5-{[4-{[(1S)-2-hydroxy-1-phenylethyl]amino}-5-(1,3,4-oxadiazol-2-yl)pyrimidin-2-yl]amino}-3,3-dimethyl-2-benzofuran-1(3H)-one 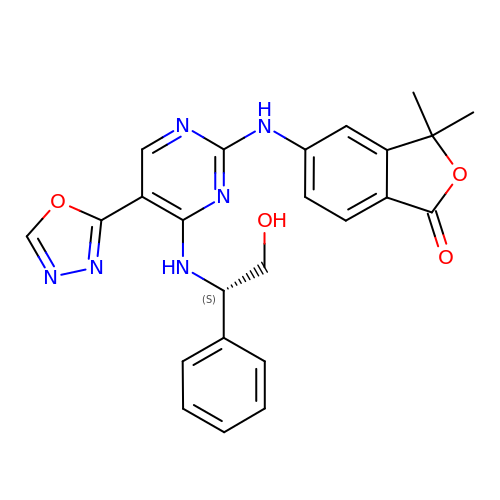| C24 H22 N6 O4 | RVSSNRBUPQUIEG-LJQANCHMSA-N>GHHHHHHAMSMQDTLLTLDTPAAVIDLDRMQRNIARMQQRMDAQGVRLRPHVKTSKSVPVAAAQRAAGASGITVSTLKEAEQFFAAGTTDILYAVSMAPHRLPQALQLRRRGCDLKLIVDSVAAAQAIAAFGREQGEAFEVWIEIDTDGHRSGVGADDTPLLLAIGRTLHDGGMRLGGVLTHAGSSYELDTPEALQALAERERAGCVQAAEALRAAGLPCPVVSVGSTPTALAASRLDGVTEVRAGVYVFFDLVMRNIGVCAAEDVALSVLATVIGHQADKGWAIVDAGWMAMSRDRGTARQKQDFGYGQVCDLQGRVMPGFVLTGANQEHGILARADGAAEADIATRFPLGTRLRILPNHACATGAQF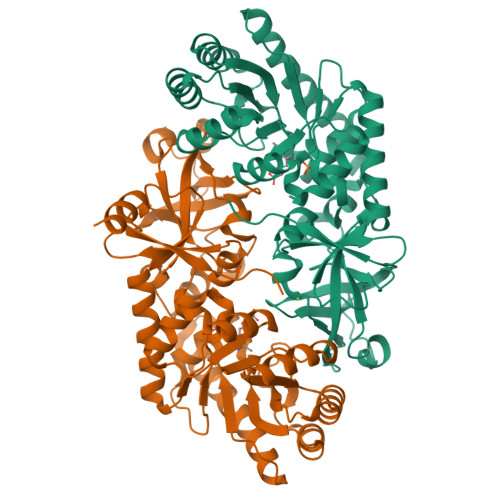PAYQALAADGSVQTWERLHGW[2x]> GCCCACCACGG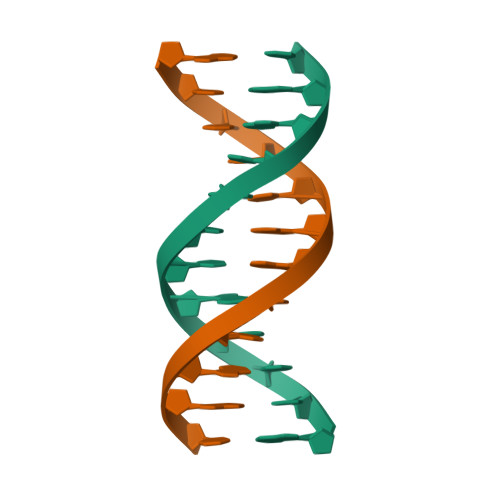C;> GCCGTGGTGGGC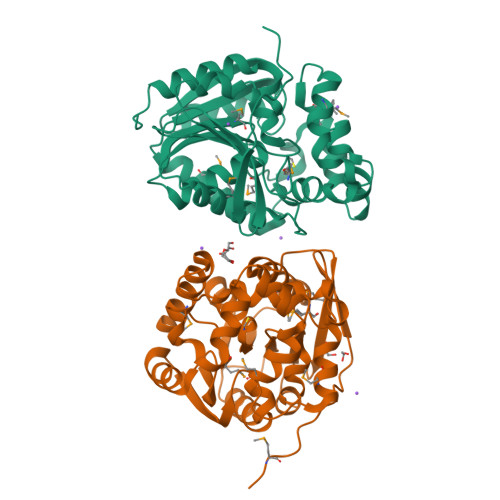>MGHHHHHHSHMAEIGTGFPFDPHYVEVLGERMHYVDVGPRDGTPVLFLHGNPTSSYVWRNIIPHVAPTHRCIAPDLIGMGKSDKPDLGYFFDDHVRFMDAFIEALGLEEVVLVIHDWGSALGFHWAKRNPERIKGIAFMEFIRPIPTWDEWPEFARETFQAFRTTDVGRKLIIDQNVFIEGTLPMGVVRPLTEVEMDHYREPFLNPVDREPLWRFPNELPIAGEPANIVALVEEYMDWLHQSPVPKLLFWGTPGVLIPPAEAARLAKSLPNCKAVDIGPGLNLLQEDNPDLIGSEIARWLSTLEISG[2x]>MLSRRYAAKSFVEWYYRQINENKPVASGYVNNNATYTKAGHPPADITINGRVVATPEEWDTMLKEQRAQHNTSSSSTLPIGRKPVRYDVDCFDVHVINADYRFAAPQRMIEQHAPTDGVRMMMALTVSGSVYFGASPRSTDDYVIKQHF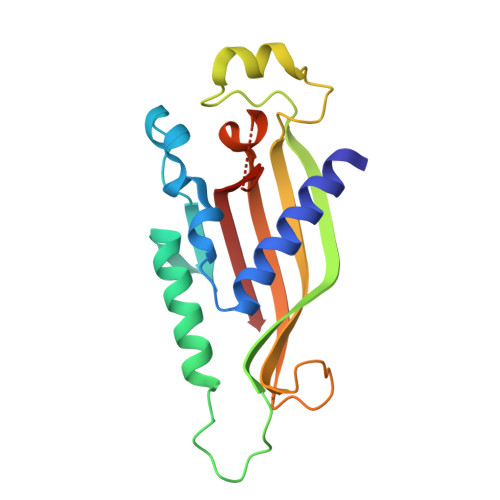NDVFILVPNWDVLEKPGARSGRKYLIASHKYRAY[2x]>[9x]MSKITVKSPGRVNLIGEHTDYTYGYVMPMAIDLYTIITAEKYDKVQLYSEHFNEEKTFTLDNLTKEGSWIDYVKGVLWVLIQEGYKIGGLKGKITGDLPLGAGLSSSASFEVGILEVLNQLYNLNIDPLKKALLAKKAENEFVGVPCGILDQFAVVFGKKDNV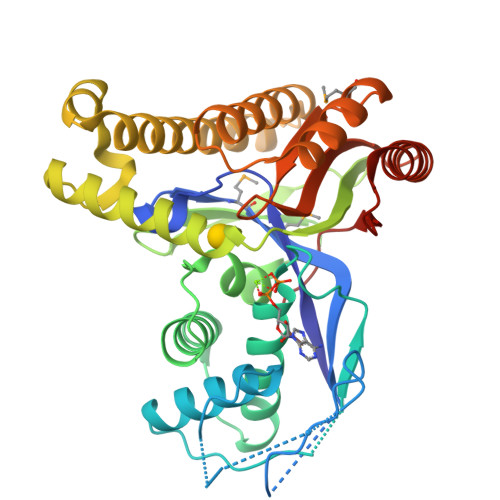IFLDTQTLQYEYIPFPKDVSVLVFYTGVKRELASSEYAERKRIAEESLRILGKESSKEVTEKDLGKLPPLHRKFFSYIVRENARVLEVRDALKEGDIEKVGKILTTAHWDLAENYRVSCEELDFFVKKAMELGAYGARLTGAGFGGSAIALVDKDKAKTIGDAILREYLAKFSWKAKYFVVKPSDGVGV>[2x]GAMDPEFPSLEQDDEDEETRMVIVGKISFCPKDVLGHGAEG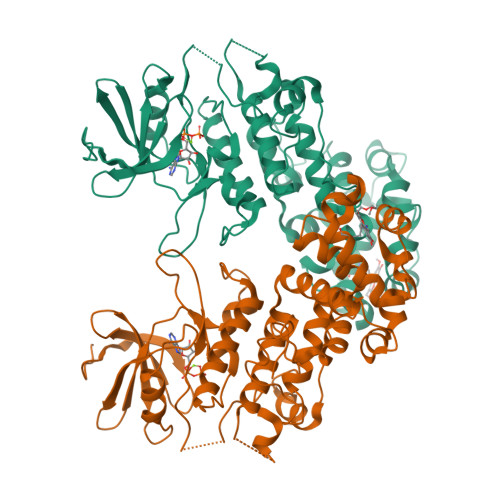TIVYKGMFDNRDVAVKRILPECFSFADREVQLLRESDEHPNVIRYFCTEKDRQFQYIAIELCAATLQEYVEQKDFAHLGLEPITLLHQTTSGLAHLHSLNIVHRDLKPHNILLSMPNAHGRIKAMISDFGLCKKLAVGRHSFSRRSGVPGTEGWIAPEMLSEDCKDNPTYTVDIFSAGCVFYYVISEGYHPFGKSLQRQANILLGACNLDCFHSDKHEDVIARELIEKMIAMDPQQRPSAKHVLKHPFFWSLEKQLQFFQDVSDRIEKEALDGPIVRQLERGGRAVVKMDWRENITVPLQTDLRKFRTYKGGSVRDLLRAMRNKKHHYRELPVEVQETLGSIPDDFVRYFTSRFPHLLSHTYQAMELCRHERLFQTYYWHEPTEPQPPVIPYAL> MSSDPFKKVERDYHNERSVHKHFASYPLKFWWGLNKFETIQGIHSILGNA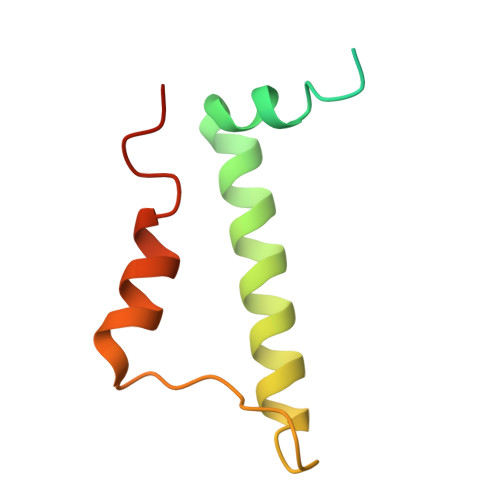ADLVVSTLSFIPGVQGRNNASYIENSIRVTRFRGFDDKTQ> MNGVYDVGGTDGLGPINRPADEPVFRAEWEKVAFAMFPATFRAGFMGLDEFRFGIEQMNPAEYLE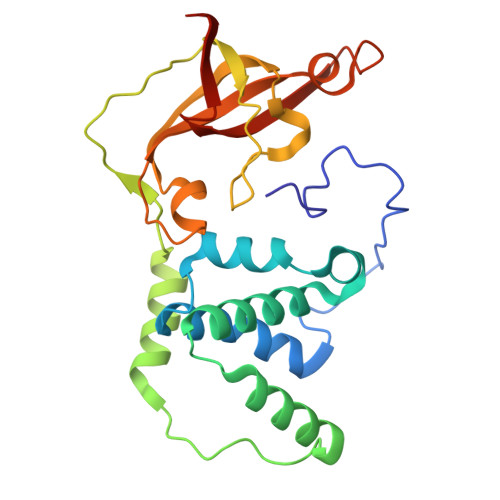SPYYWHWIRTYIHHGVRTGKIDLEELERRTQYYRENPDAPLPEHEQKPELIEFVNQAVYGGLPASREVDRPPKFKEGDVVRFSTASPKGHARRARYVRGKTGTVVKHHGAYIYPDTAGNGLGECPEHLYTVRFTAQELWGPEGDPNSSVYYDCWEPYIELVDTKAAAA> GEEEVPGNVRNGIVLNVTDTGIISNEPSTRTEDTGFVTTFTQGDQIGLFAVKDGAILDEINNMPFTFNGSSWSGKPILYDDRLVGVNFYAYYPYQSEMTGKTDLIGDDFFAPLAAGWELTTEQSDQKAYAKQDLMTSNATALIGENGNYSLSFQLTHRMSLVVVKLPSTRYIFTDAEGVAMPEETPYVAM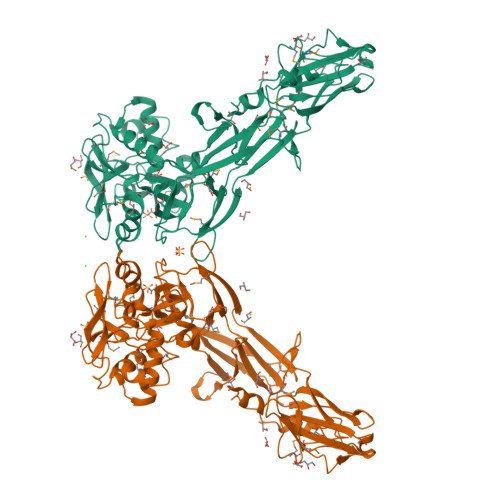SVDVAFYLDNVEEGTKISPYYDAKKDEYRLLRKPSSENQIIGHYNDKQCTLDTAEKMKEGKYKRFVVDGGYKEVTHHLQVGDYYYADGSVVSGNEAEPAKDNCIGIVCWVGNPMPSVLYKDVAGTPYTATNDALLRSHPNCVHGLVMSLYTETGKFSPALTQSIHDWFMTTSFTSSYVSVTGYYDANENNKNKPLRFLGYNNSEVLDLYYDTFKTDFECFQYQDDCESSFPSPSITTGWYVPSSGELVALQDKDNSLESKLNTKLIKVSDKTMDISATYWSSTERNNKNMYIVTYSKTAGSAGTGGVKTNTYTYRFFLGF> MLTIDYNSYRTTTPYGKRVRFLVLHYTAL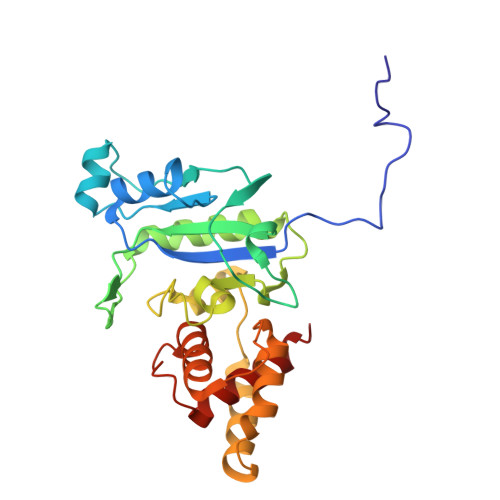DFAASVKALTTGAASAHYLIPAPHDPSYKAAGFKGQRIFNLVAEEDRAWHAGVSGWARRDNLNDTSIGIEIVNLARDDDGVFTFPDYERSQINALKQLAKNILQRYPDMTPKNVVGHSDIAVGRKSDPGPKLPWKELYEAGIGAWYDDATRDRYREGFERDGLPPRADLLEAFRLYGYALPATVDDAYFASLLRAFQMHFRPENYDGALDVETAAILYALNEKYPA> MKRVMVIGGDGYCGWATALHLSKKNYEVCIVDNLVRRLFDHQLGLESLTPIASIHDRISRWKALTGKSIELYVGDICDFEFLAESFKSFEPDSVVHFGEQRSAPYSMIDRSRAVYTQHNNVIGTLNVLFAIKEFGEECHLVKLGTMGEYGTPNIDIEEGYITITHNGRTDTLPYPKQASSFYHLSKVHDSHNIAFTCKAWGIRATDLNQGVVYGVKTDETEMHEELRNRLDYDAVFGTALNRFCVQAAVGHPLTVYGKGGQTRGYLDIRDTVQCVEIAIANPAKAGEFRVFNQFTEQFSVNELASLVTKAGSKLGLDVKKMTVPNPRVE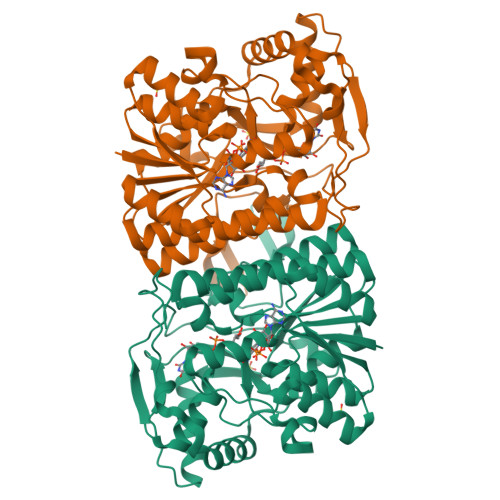AEEHYYNAKHTKLMELGLEPHYLSDSLLDSLLNFAVQFKDRVDTKQIMPSVSWKKIGVKTKSMTT> GPLGSVEQELATKMLQIQSKRFYLDVKQNRRGRFIKVAEIGADGRRSQIYLALSTAAEFRDHLSSFSDYYASLGPPNTDNLPEDGKLKSEMMIKDYRRYYLDLKENARGRFLRVSQTITRGGPRSQIALPAQGMIEFRDALTDLLEEFGAND

Pur-alpha is an ubiquitously expressed, multifunctional protein that binds to both DNA and RNA and is known to regulate replication, transcription, and translation. It has been shown that Pur-alpha binds to single- and double-stranded nucleic acids that contain GGN motifs. Nucleic acid-binding of Pur-alpha is mediated by three central PUR repeats, which are N-terminally flanked by unstructured, glycine-rich sequences and C-terminally by glutamine- and glutamate-rich regions (Johnson et al., 2013). Besides its ability to bind RNA and DNA, Pur-alpha possesses dsDNA-destabilizing activity in an ATP-independent fashion.

We present the co-crystal structure of Pur-alpha with a CGG trinucleotide-repeat DNA, providing a detailed structural explanation for nucleotide recognition. Crystals of Pur-alpha repeat I-II with a GCGGCGG trinucleotide-repeat ssDNA diffracted to a resolution of 2.0 Å. The DNA-bound protein shows the typical intramolecular dimer with two PUR repeats tightly intertwined with each other, forming a globular PUR domain (Graebsch et al., 2009). In the crystal structure, the DNA molecule 1 (DNA 1) is clamped between residues of PUR repeat I and II. PUR repeat II binds DNA 1 with the residue K138 of its β-sheet, and residues N140 and R142 of the short linker, whereas PUR repeat I contacts the DNA 1 via residues Q52, S53, and K54 in its short linker. Pur-alpha mainly binds to stacking guanine bases, but also to one of the cytosines (C5) and to the sugar phosphate backbone. Instead, F145 from the β-sheet of PUR repeat II stacks with the neighboring guanine G4 and thereby blocks the space for the cytosine C5. F145 of Pur-alpha shows particularly unusual characteristics by undergoing aromatic stacking with G4. This protein-DNA interaction blocks additional DNA-base stacking events and forces the DNA to flip out its cytosine base (C5), leading to a strong twist of the DNA 1 strand. In the crystal structure, an additional DNA-binding event was observed for PUR repeat I. The residues Y57, D59, K61, K70, and R80 of the β-sheet interact with the 3’-end of the second DNA molecule (DNA 2). All other mutations showed reduced DNA binding and only decreased unwinding. Together these observations suggest that the heterotypic stacking of DNA-bases with F145 in PUR repeat II stabilizes the single-stranded conformation of DNA and enforces a twist of the bases that is important for its unwinding activity.>[8x]DLPGLQGATRICTPQGKGLKRLSEGDLAIIDAPDLSRTFAQRLLAAKPAAVLNVSRFTTGSVPNFGPQMLIDGGIQLVEGFGQELLDGTKDGKKGRLTEDGQLFYGERLISNGSVLSGPAAENAFADAQQSLLDRMEAYFG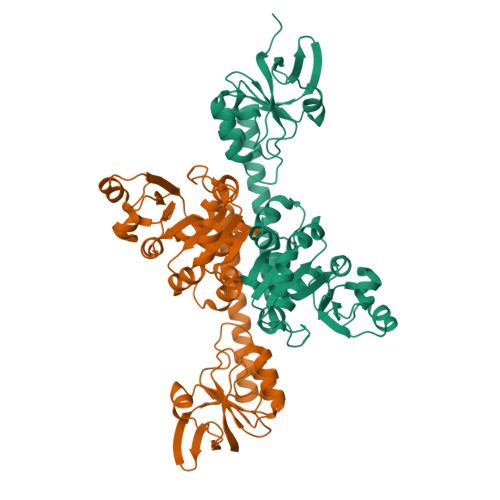NTIQFIHSEAPLLIDGLGIPDTGNAIEGRKVLIASPGDNHRSRLKELRSFIREYDPVLIGVDGAADTLVELGYKPALIVGNPTGIGADALRSGANVILPADPDGHAVGLERIQDLGIGAMTFPSSVNSSTDLALLLADFHNPQMIVNVGGPVTLDGVFENREDSDPAALLTRAKLGTKLVDGSVIASLYTVR2-(2,6-difluoro-4-methoxyphenyl)-1-(4-{4-[(3-methyl-1H-pyrazol-5-yl)amino]pyrrolo[2,1-f][1,2,4]triazin-2-yl}piperazin-1-yl)ethanone 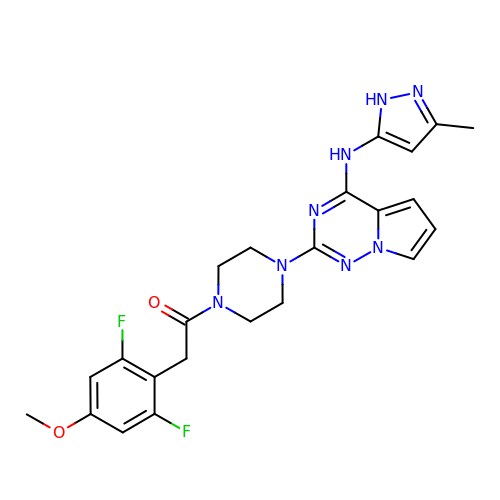| C23 H24 F2 N8 O2 | CFXACTJFCDMPJK-UHFFFAOYSA-N>[2x]MEKRMSTQQRAAGNACPTAAFSFDPARLAQRRRWAGAFAALCGLALSPSALLAEEHSQHQDHAVELAPSVVTGVAQSSPLTIVTNPKEPRQPVPASDGADYLKTIPGFAVIRNGGSNGDPVLRGMFGSRLNILTNGGMMLGAAPNRMDAPTSYISPETYDKLTVIKGPQTVLWGPGASAGTILFEREPERFGELGSRVNASLLAGSNGRFDKVLDAAAGNRLGYLRFTGNHAQSDDYEDGAGN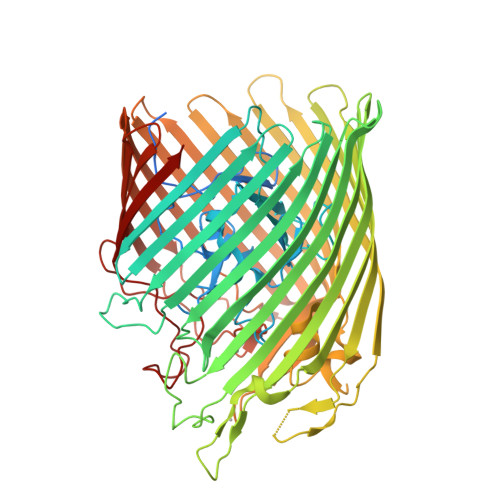TVPSRWKKWNGDVAVGWTPDEDTLIELTAGKGDGEARYAGRGMDGSQFKRESLGLRFVKSNVSDVLEKVEAQVYYNYADHIMDNFRLRTPDPSSMMPMPMASQVDRRTLGGRLAATWRWDDFKLVTGVDAMRNEHRARGSKYDMMTDYYTDADQFPWSKDAVFHNYGAFGELTWFAAERDRLIGGLRLDRASVKDYRQTLKSGHMGHAMANPTANDTRADTLPSGFVRYEHDLADSPTTLYAGLGHAERFPDYWELFSPKRGPNGSVNAFDKIKPEKTTQLDFGLQYNGDKLQAWASGYVGVVQDFILFSYREGMMGSSTQATNVDARIMGGELGASYQLTGNWKTDASLAYAWGKNSSDDRALPQIPPLEARFGLTYEEGDWSAGSLWRVVAPQNRIARDQGNVVGKDFDKSAGFGVFSLNGAYRVTRNVKLSAGVDNLFDKDYTEHLNKAGDAGFGFSANETVPEPGRTFWTKVDFSF>[4x]MKILVIEDDALLLQGLILAMQSEGYVCDGVSTAHEAALSLASNHYSLIVLDLGLPDEDGLHFLSRMRREKMTQPVLILTARDTLEDRISGLDTGADDYLVKPFALEELNARIRALLRRHNNQGDNEISVGNLRLNVTRRLVWLGETALDLTPKEYALLSRLMMKAGSPVHREILYNDIYSGDNEPATNTLEVHIHNLREKIGKSRIRTVRGFGYMLANNDDTEHLEHHHHHH

The PmrA/PmrB TCS is a major regulator of genes for lipopolysaccharide modification in the outer membrane of bacteria. The response regulator PmrA, which belongs to the OmpR/PhoB family, functions as a transcription factor. Each OmpR/PhoB member contains an N-terminal receiver domain (REC) and a C-terminal DNA-binding domain (DBD), connected by a linker. Here, we determine the crystal structure of BeF3−-activated PmrA in complex with the promoter DNA, which also reveals a REC–DBD interface in the upstream protomer, but the interactions of the interface are notably different from those observed in the KdpE–DNA complex structure.

We reveal the crystal structures of BeF3−-activated PmrA in complex with 25-bp DNA at 3.2 Å resolution and with 26-bp DNA at 3.8 Å resolution. The space group of the PmrA–25-bp DNA crystal is C222, with two copies of the protein–DNA complex (complex-1 and complex-2) in the asymmetric unit. Complex-1 structure, with the highest resolution and lowest r.m.s.d. as compared with the other two complex structures, was selected as the representative PmrA–DNA complex structure. When superimposing all Cα coordinates of the PmrA dimer between the three complex structures, complex-2 exhibited the largest root mean square deviation (r.m.s.d.), 2.2 Å. In complex-2, PmrA-2 DBD interacts with the PmrA-1 REC in the symmetric unit, possibly causing the conformational deviation for complex-2. In complex-1, the two RECs form a twofold symmetrical dimer, whereas the two DBDs bind to DNA in a head-to-tail orientation. The interface between PmrA-1 and PmrA-2 is 1,336 Å2, with the two RECs contributing to 1,024 Å2. The two DBDs fit complementarily to each other with an interface of 291.8 Å2 in complex-1. In PmrA-2, the REC and DBD are linked by an extended linker without any interdomain interaction. Interestingly, in PmrA-1, the linker forms a turn-like conformation stabilized by an H-bond and a salt bridge interaction, and REC and DBD exhibit extensive contacts via an interface of 702 Å2, with 11 H-bond interactions identified between residues from the N terminus, α1–β2 loop, α2–β3 loop, α5 of REC and side chains from α6, α7, and transactivation loop of DBD.[[(2S,3S,4R,5S)-5-(3-aminocarbonylpyridin-1-ium-1-yl)-3,4-bis(oxidanyl)oxolan-2-yl]methoxy-oxidanyl-phosphoryl] [(2S,3S,4R,5S)-5-(4-azanyl-2-oxidanylidene-pyrimidin-1-yl)-3,4-bis(oxidanyl)oxolan-2-yl]methyl 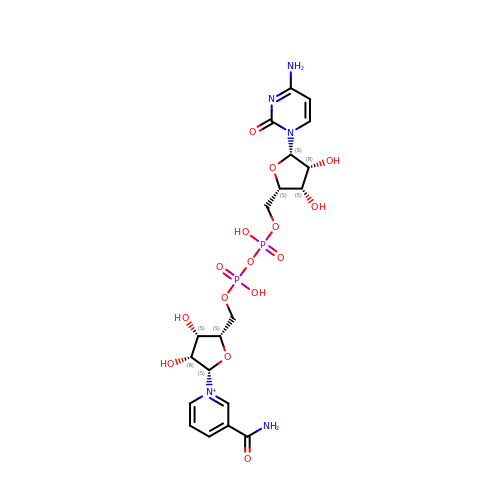hydrogen phosphate | C20 H28 N5 O15 P2 | CRWNYXSXULHVKY-JKHXZYGESA-O>HMASMRISSLTLGLVDTNTYFIENDKAVILIDPSGESEKIIKKLNQINKPLKAILLTHAHFDHIGAVDDIVDRFDVPVYMHEAEFDFLKDPVKNGADKFKQYGLPIITSKVTPEKLNEGSTEIEGFKFNVLHTPGHSPGSLTYVFDEFAVVGDTLFNNGIGRTDLYKGDYETLVDSIQDKIFELEGD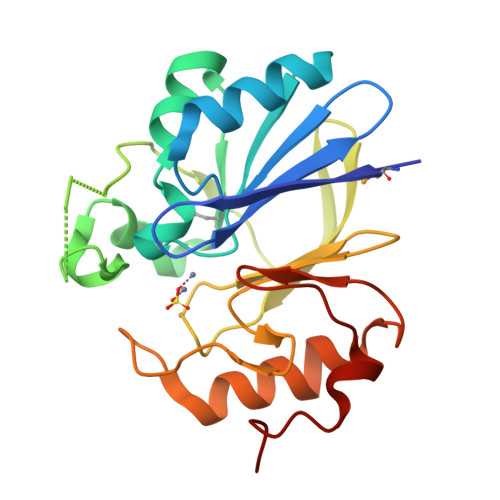LPLFPGHGPYTTVDDEQLNPFLHG[4x]> AERPTLPIPDLLTTDARNRIQLTIGAGQSTFGGKTATTWGYNGNLLGPAVKLQRGKAVTVDIYNQLTEETTLHWHGLEVPGEVDGGPQGIIPPGGKRSVTLNVDQPAATCWFHPHQHGKTGRQVAMGLAGLVVIEDDEILKLMLPKQWGIDDVPVIVQDKKFSADGQIDYQLDVMTAAVGWFGDTLLTNGAIYPQHAAPRGWLRLRLLNGCNARSLNFATSDNRPLYVIASDGGLLPEPVKVSELPVLMGERFEVLVEVNDNKPFDL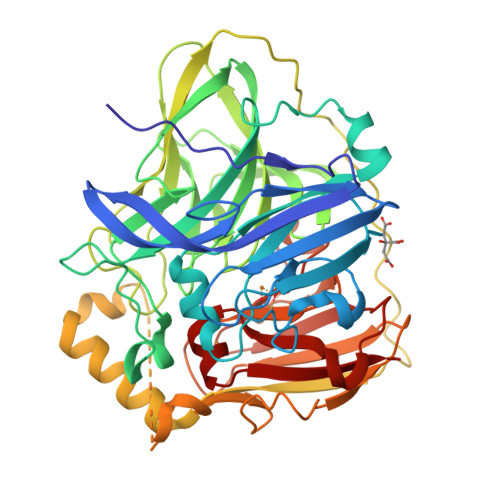VTLPVSQMGMAIAPFDKPHPVMRIQPIAISASGALPDTLSSLPALPSLEGLTVRKLQLSMDPMLDMMGMQMLMEKYGDQAMAGMDHSQMMGHMGHGNMNHMNHGGKFDFHHANKINGQAFDMNKPMFAAAKGQYERWVISGVGDMMLHPFHIHGTQFRILSENGKPPAAHRAGWKDTVKVEGNVSEVLVKFNHDAPKEHAYMAHCHLLEHEDTGMMLGFTVG> LVHVASVEKGRSYEDFQKVY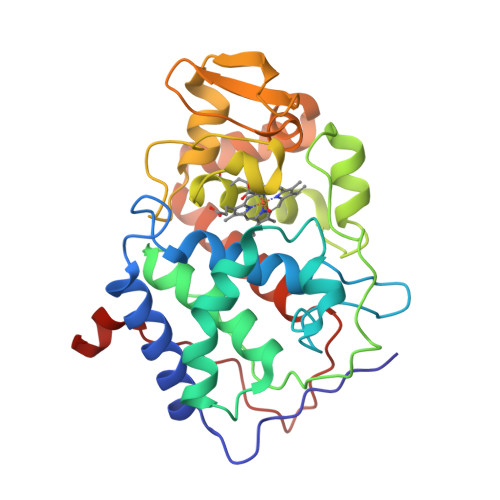NAIALKLREDDEYDNYIGYGPVLVRLAWHISGTWDKHDNTGGSYGGTYRFKKEFNDPSNAGLQNGFKFLEPIHKEFPWISSGDLFSLGGVTAVQEMQGPKIPWRCGRVDTPEDTTPDNGRLPDADKDAGYVRTFFQRLNMNDREVVALMGAHALGKTHLKNSGYEGPWGAANNVFTNEKYLNLLNEDWKLEKNDANNEQWDSKSGYMMLPTDYSLIQDPKYLSIVKEYANDQDKFFKDFSKAFEKLLENGITFPKDAPSPFIFKTLEEQGL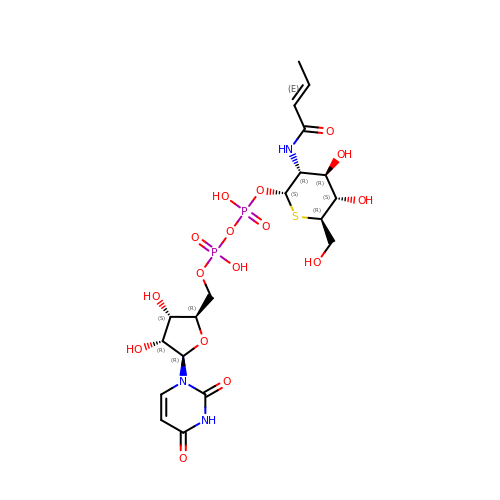(2S,3R,4R,5S,6R)-3-[(2E)-but-2-enoylamino]-4,5-dihydroxy-6-(hydroxymethyl)tetrahydro-2H-thiopyran-2-yl [(2R,3S,4R,5R)-5-(2,4-dioxo-3,4-dihydropyrimidin-1(2H)-yl)-3,4-dihydroxytetrahydrofuran-2-yl]methyl dihydrogen diphosphate (non-preferred name) | C19 H29 N3 O16 P2 S | AFVRCJQTNTUWNQ-PIXURASRSA-N> SLTFYPAWLTVSEGANATFTCSLSNWSEDLMLNWNRLSPSNQTEKQAAFSNGLSQPVQDARFQIIQLPNRHDFHMNILDTRRNDSGIYLCGAISLHPKAKIEESPGAELVVTERILE;> MLFTVTAPKEVYTVDVGSSVSLECDFDRRECTEL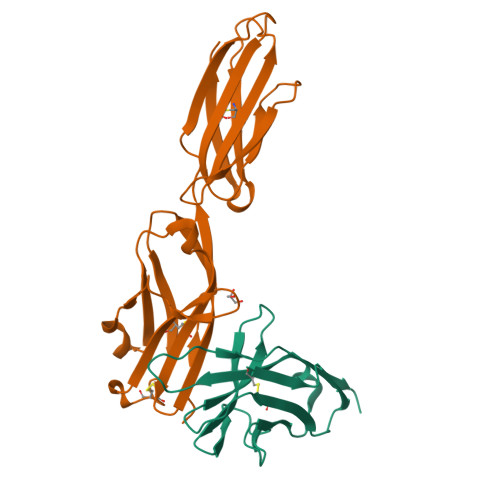EGIRASLQKVENDTSLQSERATLLEEQLPLGKALFHIPSVQVRDSGQYRCLVICGAAWDYKYLTVKVKASYMRIDTRILEVPGTGEVQLTCQARGYPLAEVSWQNVSVPANTSHIRTPEGLYQVTSVLRLKPQPSRNFSCMFWNAHMKELTSAIIDPLSRMEPKVPRT>KNRDMPLDSDVFRVPPGYNAPQQVHITQGDLVGRAMIISWVTMDEPGSSAVRYWSEKNGRKRIAKGKMSTYRFFNYSSGFIHHTTIRKLKYNTKYYYEVGLRNTTRRFSFITPPQTGLDVPYTFGLIGDLGQSFDSNTTLSHYELSPKKGQTVLFVGDLSYADRYPNHDNVRWDTWGRFTERSVAYQPWIWTAGNHEIEFAPEINETEPFKPFSYRYHVPYEASQSTSPFWYSIKRASAHIIVLSSYSAYGRGTPQYTWLKKELRKVKRSETPWLIVLMHSPLYNSYNHHFMEGEAMRTKFEAWFVKYKVDVVFAGHVHAYERSERVSNIAYKITNGLCTPVKDQSAPVYITIGDAGNYGVIDSNMIQPQPEYSAFREASFGHGMFDIKNRTHAHFSWNRNQDGVAVEADSVWFFNRHWYPVDDST[3x];> KNRDMPLDSDVFRVPPGYNAPQQVHITQGDLVGRAMIISWVTMDEPGSSAVRYWSEKNGRKRIAKGKMSTYRFFNYSSGFIHHTTIRKLKYNTKYYYEVGLRNTTRRFSFITPPQTGLDVP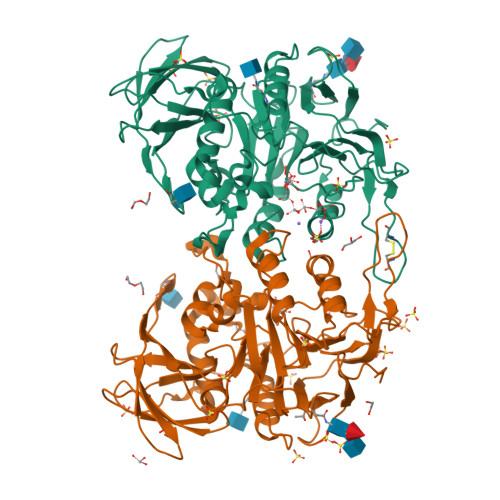YTFGLIGDLGQSFDSNTTLSHYELSPKKGQTVLFVGDLSYADRYPNHDNVRWDTWGRFTERSVAYQPWIWTAGNHEIEFAPEINETEPFKPFSYRYHVPYEASQSTSPFWYSIKRASAHIIVLSSYSAYGRGTPQYTWLKKELRKVKRSETPWLIVLMHSPLYNSYNHHFMEGEAMRTKFEAWFVKYKVDVVFAGHVHAYERSERVSNIAYKITNGLCTPVKDQSAPVYITIGDAGDYGVIDSNMIQPQPEYSAFREASFGHGMFDIKNRTHAHFSWNRNQDGVAVEADSVWFFNRHWYPVDDST>[2x]MHHHHHHMTSVMSHEFQLATAETWPNPWPMYRALRDHDPVHHVVPPQRPEYDYYVLSRH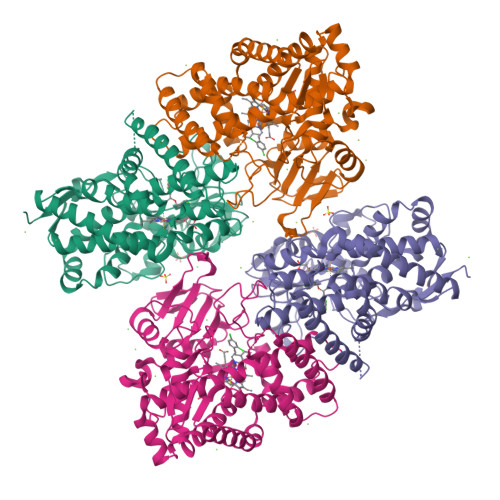ADVWSAARDHQTFSSAQGLTVNYGELEMIGLHDTPPMVMQDPPVHTEFRKLVSRGFTPRQVETVEPTVRKFVVERLEKLRANGGGDIVTELFKPLPSMVVAHYLGVPEEDWTQFDGWTQAIVAANAVDGATTGALDAVGSMMAYFTGLIERRRTEPADDAISHLVAAGVGADGDTAGTLSILAFTFTMVTGGNDTVTGMLGGSMPLLHRRPDQRRLLLDDPEGIPDAVEELLRLTSPVQGLARTTTRDVTIGDTTIPAGRRVLLLYGSANRDERQYGPDAAELDVTRCPRNILTFSHGAHHCLGAAAARMQCRVALTELLARCPDFEVAESRIVWSGGSYVRRPLSVPFRVTSSR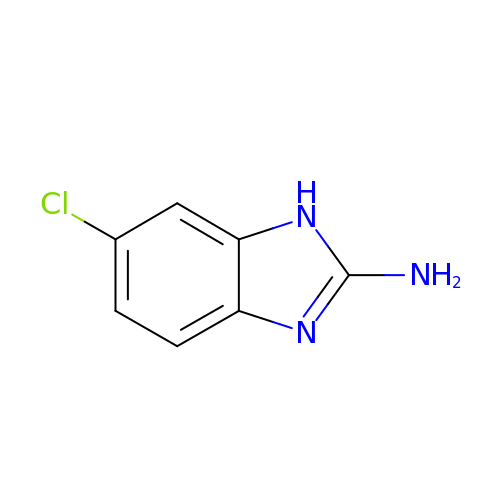6-chloro-1H-benzimidazol-2-amine | C7 H6 Cl N3 | PDOCNPCPPLPXRV-UHFFFAOYSA-N> MTKEEGRTYFESLCEEEQSLQ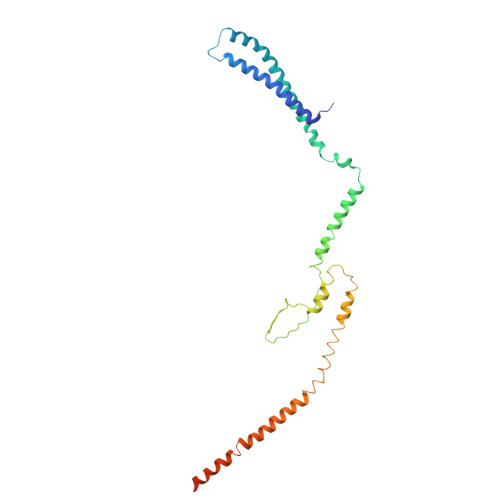ESQTHLLNILDILSVLADPRSSDDLLTESLKKLPDLHRELINSSIRLRYDKYQTREAQLLEDTKTGRDVAAGVQNPKSISEYYSTFEHLNRDTLRYINLLKRLSVDLAKQVEVSDPSVTVYEMDKWVPSEKLQGILEQYCAPDTDIRGVDAQIKNYLDQIKMARAKFGLENKYSLKERLSTLTKELNHWRKEWDDIEMLMFGDDAHSMKKMIQKIDSLKSEINAPSESYPVDKEGDIVLE>LKCNKLIPLAYKTCPAGKNLCYKMFMVSNKTVPVKRGCIDVCPKNSLLVKYVCCNTDRCN[6x]

Cobra cytotoxins (CTs) belong to the three-fingered protein family and possess membrane activity. Three-finger toxins (TFTs) are disulfide-rich proteins from the venoms of cobras, kraits, coral, and some other snakes. Their fold features three distinct β-structural “fingers”, emerging from a globular core stapled by four conserved disulfide bridges. Cardiotoxins, or cytotoxins (CTs), are one of the largest groups of TFTs, affecting the integrity of lipid membranes, and/or influencing the activity of membrane proteins and the associated signaling cascades. For the first time, a spatial model of CT13Nn with both “water” and “membrane” conformations of the central loop (loop-2) were determined by X-ray crystallography.

Structures of hexagonal (with three molecules in the asymmetric unit denoted A, B, and C) and orthorhombic (with six molecules in an asymmetric unit denoted A, B, C, D, E, and F) crystal forms were solved at 2.3 and 2.6 Å-resolution, respectively. The electron density for molecules D, E, and F of the orthorhombic structure is considerably poorer than for three other molecules, which is also reflected in the higher B-factor. RMSD for Cα atoms of molecule A of the orthorhombic structure superimposed on the other five molecules ranges from 0.39 to 1.45 Å. Significant difference between E subunit of the orthorhombic structure and most other subunits could be explained by an unusual conformation of loop-2 in all subunits, except E. Previously, this was not observed in crystal structures of homologues. Comparison of subunit E with the NMR structure of CT2Nk (in aqueous solution) showed that the conformations of the loops were very similar. Unusual conformation of the loop-2 in all subunits of the hexagonal and most subunits of the orthorhombic form was similar to that found by NMR for cytotoxin 1 from N. oxiana (5NQ4) in DPC micelle. Superimposition of the models (except E) over residues 22–36 resulted in RMSD values in the range of 0.8 to 1.1 Å. Specifically, for model E the respective RMSD value was 1.8 Å. Superimposition of subunit E and A of CT13Nn demonstrated that the tip of the loop-2 was repulsed from the hydrophobic amino acid residues 8–9 of loop-1 of the neighboring subunit B due to crystal packing. For the first time, in this work the structure similar to the membrane-bound conformation of functionally important loop-2 of an S-type CT was observed in the two crystal forms.2-aminopyrimidin-5-ol 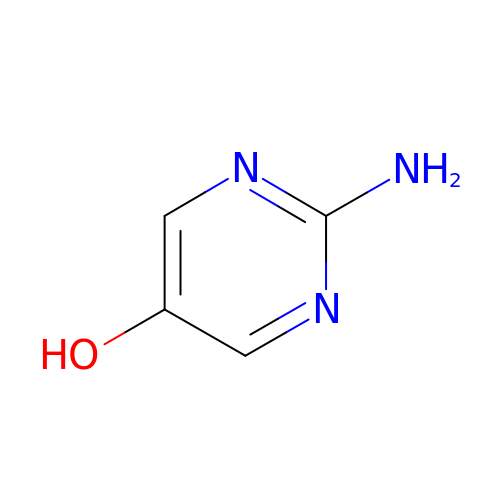| C4 H5 N3 O | NVYMOVCPYONOSF-UHFFFAOYSA-N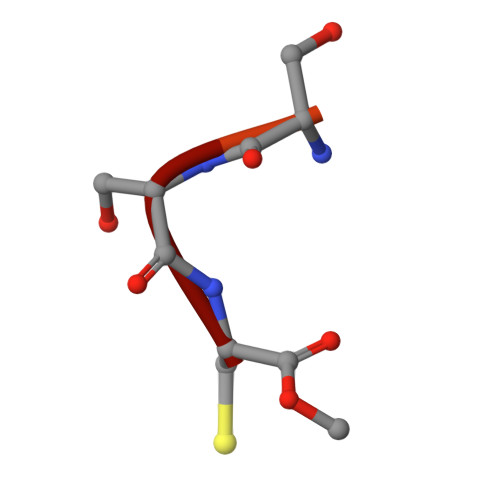> CSQQGKSSC>MKEITFKINGQEMIVPEGTTILEAARMNNIDIPTLCYLKDINEIGACRMCLVEIAGARALQAACVYPVANGIEVLTNSPKVREARRVNLELILSNHNRECTTCIRSENCELQTLATDLGVSDIPFEGEKSGKLIDDLSTSVVRDESKCILCKRCVSVCRDVQSVAVLGTVGRGFTSQVQPVFNKSLADVGCINCGQCIINCPVGALKEKSDIQRVWDAIADPSKTVIVQTAPAVRAALGEEFGYPMGTSVTGKMAAALRRLGFDKVFDTDFGADVCIMEEGTELIGRVTNGGVLPMITSCSPGWIKFIETYYPEAIPHLSSCKSPQNITGALLKNHYAQTNNIDPKDMVVVSIMPCTAKKYEVQREELCTDGNADVDISITTRELARMIKEARILFNKLPDEDFDDYYGESTGAAVIFGATGGVMEAAVRTVADVLNKKDIQEIDYQIVRGVDGIKKASVEVTPDLTVNLVVAHGGANIREVMEQLKAGELADTHFIELMACPGGCVNGGGQPIVSAKDKMDIDIRTERAKALYDEDANVLTYRKSHQNPSVIRLYEEYLEEPNSPKAHHILHTKYSAKPKLV[2x];>MAYKRSQILICGGTGCTSSGSMVLVKELKKELVKHDILDEVEVVTTGCFGLCELGPVVIVYPEGTFYSRVEAADIPEMVEEHLVKGRPLDRLIYNEKGDGHHPLSINELGFFKKQRRIALANCGVINPENIDEYIGFDGYLALEKVLLTMSPVDVINEVKASGLRGRGGGGFPTGLKWQFAHDAVSEDGIKYVACNADEGDPGAFMDRSVLEGDPHAVIEAMAIAGYAVGASKGYVYVRAEYPIAVNRLQIAIDQAKEYGILGENIFETDFSFDLEIRLGAGAFVCGEETALMNSIEGKRGEPRPRPPFPANKGLFGKPTVLNNVETYANIPKIILNGAEWFASVGTEKSKGTKVFALGGKINNTGLLEIPMGTTLREIIYEIGGGIPNGKAFKAAQTGGPSGGCLPESLLDTEIDYDNLIAAGSMMGSGGLIVMDEDNCMVDVARFFLDFTQDESCGKCPPCRIGTKRMLEILERICDGKGVEGDIERLEELAVGIKSSALCGLGQTAPNPVLSTIRFFRDEYEAHIRDKKCPAGVCKHLLDFKINADTCKGCGICAKKCPADAISGEKKKPYNIDTSKCIKCGACIEACPFGSISKA[2x];>[2x]MAELIPVENLDVVKAIVAEHREVPGCLMQILQETQLKYGYLPLELQGTIADELGIPLTEVYGVATFY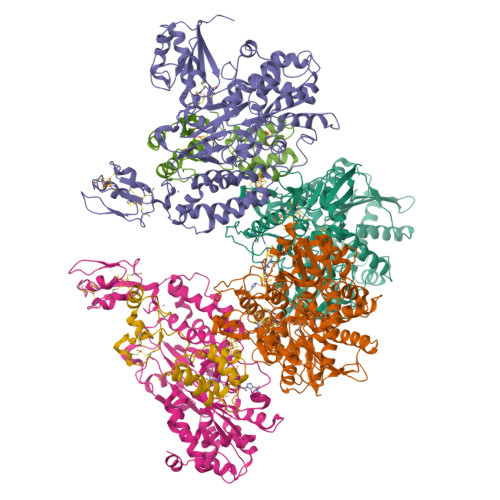SQFTLKPKGKYKIGICLGTACYVRGSQAIIDKVNSVLGTQVGDTTEDGKWSVDATRCVGACGLAPVMMINEEVFGRLTVDEIPGILEKY(1~{Z},3~{R},4~{S},7~{S},8~{Z})-8-ethylidene-4,7-bis(oxidanyl)-5-oxidanylidene-3-propyl-cyclononene-1,2-dicarboxylic acid | C16 H22 O7 | 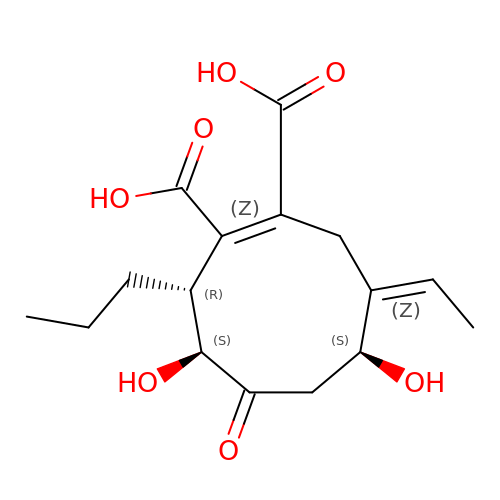YFQGJJCDYCWLSI-KRKAZGBPSA-N> RSMAAEVYFGDLELFEPFDHPGESIPKPVHTRFKDDDGDEEDENGVGDAELRERLRQCEETIEQLRAENQELKRKLNILTRPSGILVNDTKLDGPILQILFMNNAISKQYHQEIEEFVSNLVKRFEEQQKNDVEKTSFNLLPQPSSIVLEEDHKVEESCAIKNNKEAFSVVGSVLYFTNFCLDKLGQPLLNENPQLSEGWEIPKYHQVFSHIVSLEGQEIQVKAKRPKPHCFNCGSEEHQMKDCPMPRNAARISEKRKEYMDACGEANNQNFQQRYHAEEVEERFGRFKPGVISEELQDALGVTDKSLPPFIYRMRQLGYPPGWLKEAELENSGLALYDGKDGTDGETEVGEIQQNKSVTYDLSKLVNYPGFNISTPRGIPDEWRIFGSIPMQACQQKDVFANYLTSNFQAPGVKSGNKRSSSHSSPGSPKKQKNESNSAGSPADMELDSDMEVPHGSQSSESFQFQPPLPPDTPPLPRGTPPPVFTPPLPKGTPPLTPSDSPQTRTGSGAVDEDALTLEELEEQQRRIWAALEQAESVNSDSDVPVDTPLTGNSVASSPCPNELDLPVPEGKTSEKQTLDEPEVPEIFTKKSEAGHASSPDSEVTSLCQKEKAELAPVNTEGALLDNGSVVPNCDISNGGSQKLFPADTSPSTATKIHSPIPDMSKFATGITPFEFENMAESTGMYLRIRSLLKNSPRNQQKNKKASE;> GPDSMADAFGDELFSVFEGDSTTAAGTKKDKEKDKGKWKGPPGSADKAGKRFDGKLQSESTNNGKNKRDVDFEGTDEPIFGKKPRIEESITEDLSLADLMPRVKVQSVETVEGCTHEVALPAEEDYLPLKPRVGKAAKEYPFILDAFQREAIQCVDNNQSVLVSAHTSAGKTVCAEYAIALALREKQRVIFTSPIKALSNQKYREMYEEFQDVGLMTGDVTINPTASCLVMTTEILRSMLYRGSEVMREVAWVIFDEIHYMRDSERGVVWEETIILLPDNVHYVFLSATIPNARQFAEWICHLHKQPCHVIYTDYRPTPLQHYIFPAGGDGLHLVVDENGDFREDNFNTAMQVLRDAGDLAKGDQKGRKGGTKGPSNVFKIVKMIMERNFQPVIIFSFSKKDCEAYALQMTKLDFNTDEEKKMVEEVFSNAIDCLSDEDKKLPQVEHVLPLLKRGIGIHHGGLLPILKETIEILFSEGLIKALFATETFAMGINMPARTVLFTNARKFDGKDFRWISSGEYIQMSGRAGRRGMDDRGIVILMVDEKMSPTIGKQLLKGSADPLNSAFHLTYNMVLNLLRVEEINPEYMLEKSFYQFQHYRAIPGVVEKVKNSEEQYNKIVIPNEESVVIYYKIRQQLAKLGKEIEEYIHKPKYCLPFLQPGRLVKVKNEGDDFGWGVVVNFSKKSNVKPNSGELDPLYVVEVLLRCSKESLKNSATEAAKPAKP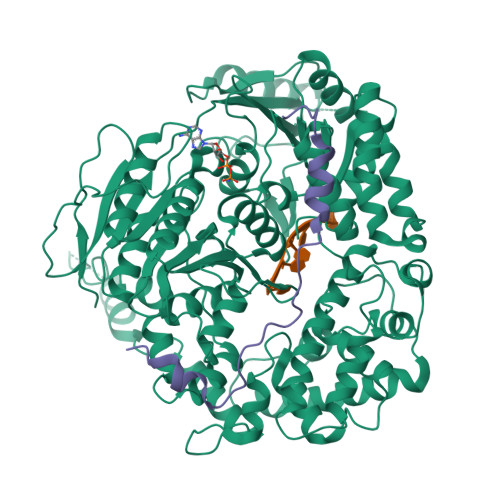DEKGEMQVVPVLVHLLSAISSVRLYIPKDLRPVDNRQSVLKSIQEVQKRFPDGIPLLDPIDDMGIQDQGLKKVIQKVEAFEHRMYSHPLHNDPNLETVYTLCEKKAQIAIDIKSAKRELKKARTVLQMDELKCRKRVLRRLGFATSSDVIEMKGRVACEISSADELLLTEMMFNGLFNDLSAEQATALLSCFVFQENSSEMPKLTEQLAGPLRQMQECAKRIAKVSAEAKLEIDEETYLSSFKPHLMDVVYTWATGATFAHICKMTDVFEGSIIRCMRRLEELLRQMCQAAKAIGNTELENKFAEGITKIKRDIVFAASLYL> QQAGTETEEYHLPLTWERDGSSVSASVVIDSNWRWTHSTEDTTNCYDGNEWDSTLCPDADTCTENCAIDGVDQGTWGDTYGITASGSKLTLSFVTEGEYSTDIGSRVFLMADDDNYEIFNLLDKEFSFDVDASNLPCGLNGALYFVSMDEDGGTSKYSTNTAGAKYGTGYCDAQCPHDMKFIAGKANSDGWTPSDNDQNAGTGEMGACCHEMDIWEANSQAQSYTAHVCSVDGYTPCTGTDCGDNGDDRYKGVCDKDGCDYAAYRLGQHDFYGEGGTVDSGSTLTVITQFITGGGGLNEIRRIYQQGGQTIQNAAVNFPGDVDPYDSITEDFCVDIKRYFGDTNDFDAKGGMSGMSNALKKGMVLVMSLWDDHYANMLWLDATYPVDSTEPGALRGPCSTDSGDPADVEANFPGSTVTFSNIKIG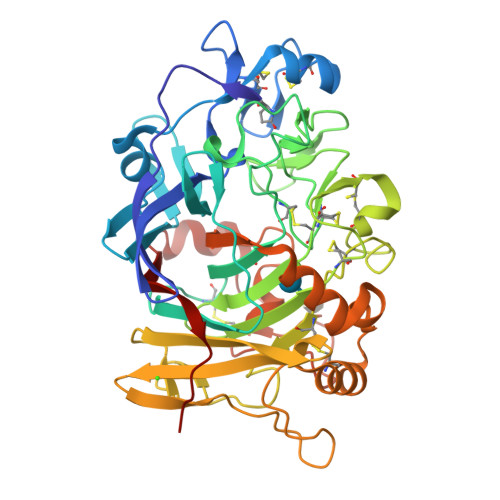PIQSYD>SMYKVILVNDDYTPMEFV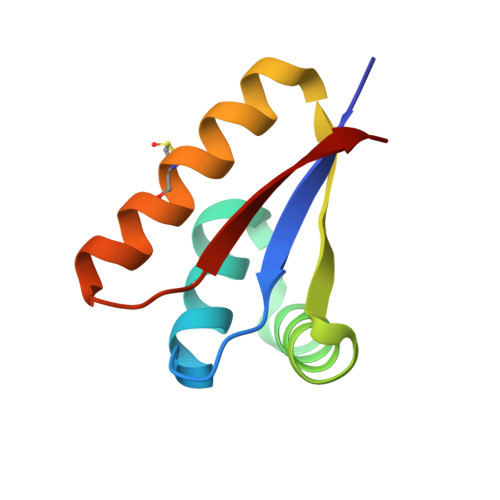IDVLQKFFSYDVERATQLMLAVHYQGKAICGVFTAEVAETKVAMVNKYARENEHPLLCTLEKA[2x]>[3x]MAKRLSKQQLAKAIANTLETPPQPKAGRRRNRRRQRSAVQQLQPTQAGISMAASAQGAMVRIRNPAVSSSRGGITVLTHSELSAEIGVTDSIVVSSELVMPYTVGTWLRGVAANWSKYSWLSVRYTYIPSCPSSTAGSIHMGFQYDMADTVPVSVNQLSNLRGYVSGQVWSGSAGLCFINGTRCSDTSTAISTTLDVSKLGKKWYPYKTSAD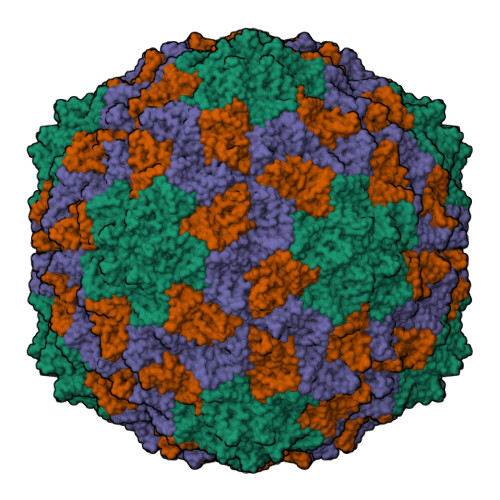YATAVGVDVNIATPLVPARLVIALLDGSSSTAVAAGRIYCTYTIQMIEPTASALNN Here, we showed three complex structures of 6mA demethylase C. elegans NMAD-1A, a canonical isoform of NMAD-1 (F09F7.7). NMAD-1, one of the AlkB family members in C. elegans, demethylates the DNA damage modification such as 6mA and 3mC. C. elegans NMAD-1A protein has 291 residues involving an N-terminal extension (NTE), a nucleotide-recognition lid (NRL), a DSBH domain, and the CTD. Like other AlkB family proteins, NMAD-1A requires the binding of the cosubstrate α-KG and ferrous iron for catalysis.

Although we finally obtained the structure of mut3 NMAD-1A1-291 full-length crystals, the ZFD exhibited poorly defined electron density. Here, we illustrate the structural features of NMAD-1A by the mut3 NMAD-1A1-291-Mn2+-α-KG structure mainly. The DSBH, as the catalytic core of NMAD-1A, adopts a typical eight-stranded (β9–β16) jelly-roll fold that contains a major sheet of antiparallel β-strands (β9–β16–β11–β14) and a minor sheet (β10–β15–β12–β13) to sandwich Mn2+ and α-KG ligands at the active center, a large α-helix α3, a small α-helix α4, and two 310 helixes (η1–η2). Additionally, the DSBH is notably wrapped around and stabilized by additional elements from the NTE, NRL, and CTD, with the NTE domain packing on one side and the NRL domain and the CTD on the opposite side. In the NMAD-1A1-291-Mn2+-α-KG complex structure, the Mn2+ ion is in an octahedral geometry and coordinated by NE2 atoms of His-184 and His-239, carboxylate oxygen of Asp-186, and the C1-carboxylate and C2-carbonyl groups of α-KG, respectively. The binding of α-KG is also apparently stabilized by hydrogen bonds with the side chains of Tyr-173, Asp-186, Ser-197, and His-239 and salt bridges involving the side chains of Arg-250 and Arg-256 in the NMAD-1A active center. Notably, the CTD interacts with and further stabilizes the Flip2 region by hydrophobic contacts, including Tyr-272, Leu-276, and Leu-279 of the CTD as well as Pro-124, Val-133, and Phe-138 of the Flip2 region. In addition, the main chains of Ile-282, Val-284, and Leu-286, together with the side chain of Tyr-272 of the CTD, form several hydrogen bonds with the main chains of Met-141, Glu-143, and Val-133 and the side chain of Glu-143 of the Flip2. In addition, SAXS analysis showed that NMAD-1A existed mainly in the form of monomer in solution. Hence, four copies of NMAD-1A found in each asymmetric unit were due to the crystal packing.

>[4x]HHHHHHENLYFQGSMGSAEQACGCKGARFCALCETTERVKKLRVVEDKHVNYKVFIYDHIRQIAIPTTNLNSQSSLEDIIDESTSCQSVSTDGSIEIDGLTLIHNFLSESEESKILNMIDTVKWAKSKSGRRKQDYGPKVNFKHKKVKTDTFVGMPEYADMLLNKMSEYDVKKLGNYQPFEMCNLEYEEVKKSAIEMHQDDMWIWGNRLISINLINGSVMTLSNDNKSFLCYVHMPHRSLLCMADECRYDWKHGVLAHHIRGRRIALTMREAAKDFAEGGELYEKYGAELIRLGNIRVPLSKTSV1-{3-[3-(1-methyl-1H-pyrazol-4-yl)isoquinolin-8-yl]-1-(oxan-4-yl)-1,4,6,7-tetrahydro-5H-pyrazolo[4,3-c]pyridin-5-yl}ethan-1-one 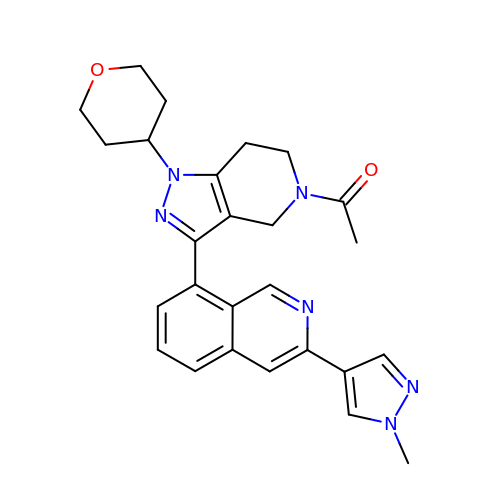| C26 H28 N6 O2 | RPDQYBNAJDAGIK-UHFFFAOYSA-N>MKPIFSRGPSLQIRLILAVLVALGIIIADSRLGTFSQIRTYMDTAVSPFYFVSNAPRELLDGVSQTLASRDQLELENRALRQELLLKNSELLMLGQYKQENARLRELLGSPLRQDEQKMVTQVISTVNDPYSDQVVIDKGSVNGVYEGQPVISDKGVVGQVVAVAKLTSRVLLICDATHALPIQVLRNDIRVIAAGNGCTDDLQLEHLPANTDIRVGDVLVTSGLGGRFPEGYPVAVVSSVKLDTQRAYTVIQARPTAGLQRLRYLLLLWGADRNGANPMTPEEVHRVANERLMQMMPQVLPSPDAMGPKLPEPATGIAQPTPQQPATGNAATAPAAPTQPAANRSPQRATPPQSGAQPPARAPGGQ[2x]

MreC is a scaffold protein required for cell shape determination through interactions with proteins related to cell wall synthesis. The periplasmic part of MreC contains a coiled‐coil domain and two six‐stranded barrel domains.

Here, we determined the crystal structure of the major periplasmic part of MreC from Escherichia coli at 2.1 Å resolution. The coiled‐coil domain is essential for dimer formation, and the two monomers are prone to relative motion that is related to the small interface of β‐barrel domains. In addition, MreC forms an antiparallel filament‐like structure along the coiled‐coil direction, which is different from the helical array structure in Pseudomonas aeruginosa. Our structure deepens our understanding of polymer formation of MreC.> MSNLSGTDKSVIL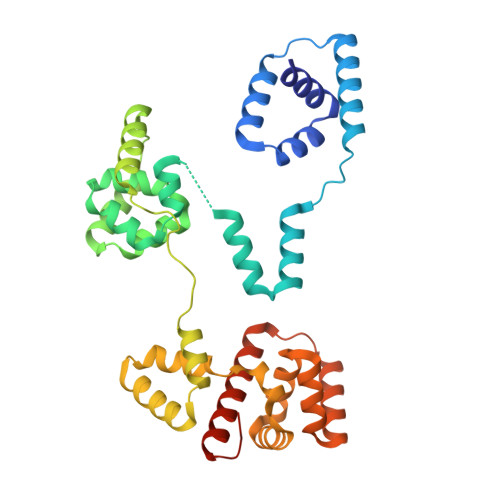LMTIGEDRAAEVFKHLSTREVQALSTAMANVRQISNKQLTDVLSEFEQEAEQFAALNINANEYLRSVLVKALGEERASSLLEDILETRDTTSGIETLNFMEPQSAADLIRDEHPQIIATILVHLKRSQAADILALFDERLRHDVMLRIATFGGVQPAALAELTEVLNGLLDGQNLKRSKMGGVRTAAEIINLMKTQQEEAVITAVREFDGELAQKIIDEMFLFENLVDVDDRSIQRLLQEVDSESLLIALKGAEPPLREKFLRNMSQRAADILRDDLANRGPVRLSQVENEQKAILLIVRRLAETGEMVIGSGEDTYV> MVK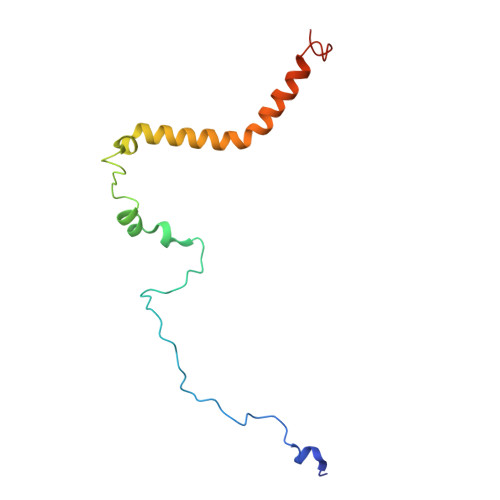TLADYIHWRNKPSSIPPVDEYRPPVPLVNYDKLSTQFFSKLDNDPVINRVLRAPKVTVMATSLPIVNHPAFLFVAGALTGFSLTYAITSHYVGRKEIENLVKFDPRYFPEYTKSS> ILVEGDGI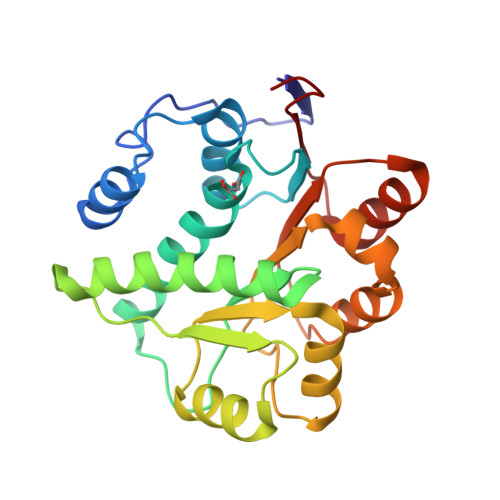PPPIKSFKEMKFPAAILRGLKKKGIHHPTPIQIQGIPTILSGRDMIGIAFTGSGKTLVFTLPVIMFCLEQEKRLPFSKREGPYGLIICPSRELARQTHGILEYYCRLLQEDSSPLLRCALCIGGMSVKEQMETIRHGVHMMVATPGRLMDLLQKKMVSLDICRYLALDEADRMIDMGFEGDIRTIFSYFKGQRQTLLFSATMPKKIQNFAKSALVKPVTINVGRAG>[2x]MPASRYITDMTIEELSRDWFMLMPKQKVEGPLCIRIDQAIMDKNIMLKANFSVIFDRLETLIL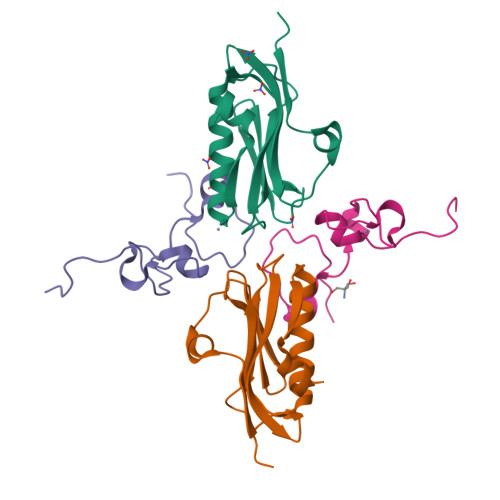LRAFTEEGAIVGEISPLPSFPGHTIEDVKNAIGVLIGGLEWNDNTVRVSKTLQRFAWGSSNENGRPPLTLEHHHHHH;>MGHHHHHHSHMSGEKTVVCKHWLRGLCKKGDQCEFLHEYDMTKMSECYFYSKFGECSNKECPFLHIDPESKI[2x]>MKILKTLTLRGPNYWSIRRKKLIVMRLDLEDLAERPSNSIPGFYEGLIKVLPSLVEHFCSPGYQGGFLERVKEGTYMGHIVEHVALELQELVGMTAGFGRTRETSTPGVYNVVYEYVDEQAGRYAGRAAVRLCRSLVDTGDYPRLELEKDLEDLRDLGANSALGPSTETIVTEAEARKIPWMLLSARAMVQLGYGVYQQRIQATLSSHSGILGVELACDKEGTKTILQDAGIPVPRGTTIQYFDDLEEAINDVGGYPVVIKPLDGNHGRGITINVRHWQEAIAAYDLAAEESKSRAIIVERYYEGSDHRVLVVNGKLVAVAERIPAHVTGDGSSTISELIEKTNQDPNRGDGHDNILTKIVVNKTAIDVMERQGYNLDSVLPKDEVVYLRATANLSTGGIAIDRTDDIHPENIWLMERVAKVIGLDIAGIDVVTSDISKPLRETNGVIVEVNAAPGFRMHVAPSQGLPRNVAAPVLDMLFPPGTPSRIPILAVTGTNGKTTTTRLLAHIYRQTGKTVGYTSTDAIYINEYCVEKGDNTGPQSAGVILRDPTVEVAVLETARGGILRAGLAFDSCDVGVVLNVAADHLGLGDIDTIEQMAKVKSVIAEVVDPSGYAVLNADDPLVAAMADKVKAKVAYFSM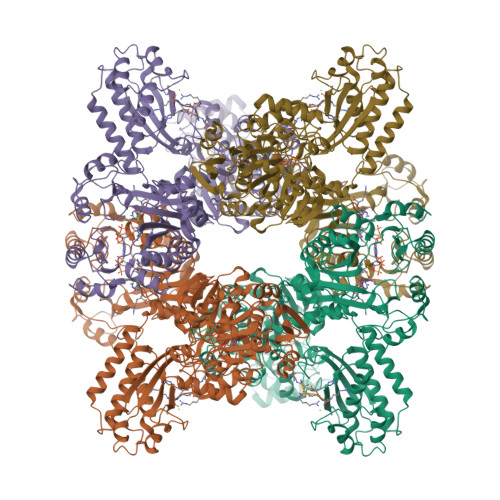NPDNPIIQAHVRRNGIAAVYESGYLSILEGSWTLRVEQAKLIPMTMGGMAPFMIANALAACLAAFVNGLDVEVIRQGVRTFTTSAEQTPGRMNLFNLGQHHALVDYAHNPAGYRAVGDFVKNWQGQRFGVVGGPGDRRDSDLIELGQIAAQVFDRIIVKEDDDKRGRSEGETADLIVKGILQENPGASYEVILDETIALNKALDQVEEKGLVVVFPESVTRAIDLIKVRNPIGENLYFQ[4x];>[8x]DDDDDDDDDDDDDDDD> MASDGVVVEIGKVTGSVGTTVEIPVYFRGVPSKGIANCDFVFRYDPNVLEIIGIDPGDIIVDPNPTKSFDTAIYPDRKIIVFLFAEDSGTGAYAITKDGVFAKIRATVKSSAPGYITFDEVGGFADNDLVEQKVSFID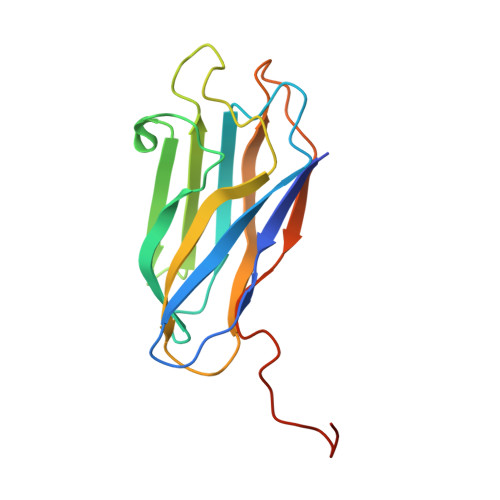GGVNVGNATPTKLEHHHHHH> ESQPDPMPDDLHKSSEFTGTMGNMKYLYDDHYVSATKVKSVDKFLAHDLIYNISDKKL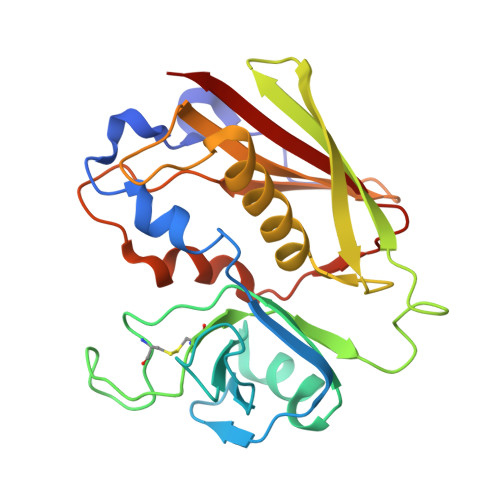KNYDKVKTELLNEDLAKKYKDEVVDVYGSNYYVNCYFSSKDNVWWHGKTCMYGGITKHEGNHFDNGNLQNVLVRVYENKRNTISFEVQTDKKSVTAQELDIKARNFLINKKNLYEFNSSPYETGYIKFIENNGNTFWYDMMPAPGDKFDQSKYLMMYNDNKTVDSKSVKIEVHLTTKNG>[2x]MRFIHALLLAGIAHSAYASEKLTFKTDLEKLEREKAAQIGVAIVDPQGEIVAGHRMAQRFAMCSTFKFPLAALVFERIDSGTERGDRKLSYGPDMIVEWSPATERFLASGHMTVLEAAQAAVQLSDNGATNLLLREIGGPAAMTQYFRKIGDSVSRLDRKEPEMSDNTPGDLRDTTTPIAMARTVAKVLYGGALTSTSTHTIERWLIGNQTGDATLRAGFPKDWVV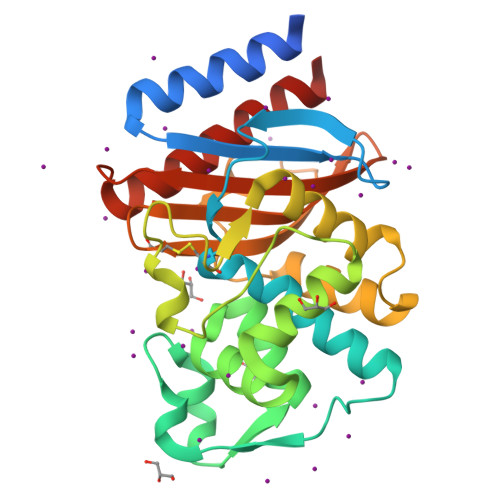GEKTGTCANGARNDIGFFKAQERDYAVAVYTTAPKLSAVERDELVASVGQVITQLILSTDK>GSGHWGAWMPSTISAFEGTCVSIPCRFDFPDELRPAVVHGVWYFNSPYPKNYPPVVFKSRTQVVHESFQGRSRLLGDLGLRNCTLLLSTLSPELGGKYYFRGDLGGYNQYTFSEHSVLDIVNTPNIVVPPEVVAGTEVEVSCMVPDNCPELRPELSWLGHEGLGEPTVLGRLREDEGTWVQVSLLHFVPTREANGHRLGCQAAFPNTTLQFEGYASLDVKYPPVIVEMNSSVEAIEGSHVSLLCGADSNPPPLLTWMRDGMVLREAVAKSLYLDLEEVTPGEDGVYACLAENAYGQDNRTVELSVMYAAAAHHHHHH[2x]

MAG is a type 1 single-pass transmembrane protein expressed on myelinating oligodendrocytes in the CNS and Schwann cells in the PNS23. Myelin-associated glycoprotein (MAG) adhesion and signalling at the myelin–axon interface regulates the formation and maintenance of myelinated axons, thus playing an important role in the development and function of the nervous system. MAG adhesion maintains the myelin–axon spacing (periaxonal diameter) by interacting with specific neuronal gangliosides (glycolipids), such as the major brain gangliosides GT1b and GD1a. On the basis of the primary sequence its extracellular region is predicted to consist of five Ig domains; an N-terminal V-type Ig domain that is typical for Siglecs and four C2-type Ig domains.

In addition, crystals of a shorter construct, consisting of the three N-terminal domains (MAG1–3), diffracted to a maximum resolution of 2.1 Å. In all three crystal forms MAG has an extended collinear conformation. Only consecutive Ig domains interact with each other via hydrophobic interfaces (buried-surface area ranging from 243 to 690 Å2) and short inter-domain linkers of up to two residues. Domains Ig1 and Ig2 form the largest interface in which the Ig2 loops at the N-terminal ‘head' side interact with the A2-B (Ig domain β–strand numbering) side of Ig1. In all three crystal forms, electron density proximal to the side chain of W22 suggests this residue is C-mannosylated. The W22-attached α-D-mannopyranosyl group has an unusual ring-flipped 1C4 chair conformation in the structures (regular mannose is 4C1). We do not observe clear electron density for any ligands in the two other crystal forms (lysine-methylated MAG1–5 and MAG1–3). In these crystal forms the unliganded MAG is apparently preferentially crystallized over the ligand-bound forms. The other glycans are not expected to interfere with dimerization, also not when considering myelin-specific N-linked glycans. We confirmed that MAG dimerizes in solution via the Ig4–Ig5 interface by analysing glycosylated and deglycosylated forms of MAG1–5, MAG1–3 (that lacks the dimerization domains) and the aforementioned mutants in small angle X-ray scattering (SAXS) and AUC experiments. Similar to the SAXS analysis, the MAG1–5 I473E and MAG1–3 SE-AUC data fit best to a single species that agrees with the Mm of a monomer.>[2x]QEDEDGDYEELVLALRSEEDGLAEAPEHGTTATFHRCAKDPWRLPGTYVVVLKEETHLSQSERTARRLQAQAARRGYLTKILHVFHGLLPGFLVKMSGDLLELALKLPHVDYIEEDSSVFAQSIPWNLERITPPRYRADEYQPPDGGSLVEVYLLDTSIQSDHREIEGRVMVTDFENVPEEDGTRFHRQASKCDSHGTHLAGVVSGRDAGVAKGASMRSLRVLNCQGKGTVSGTLIGLEFIRKSQLVQPVGPLVVLLPLAGGYSRVL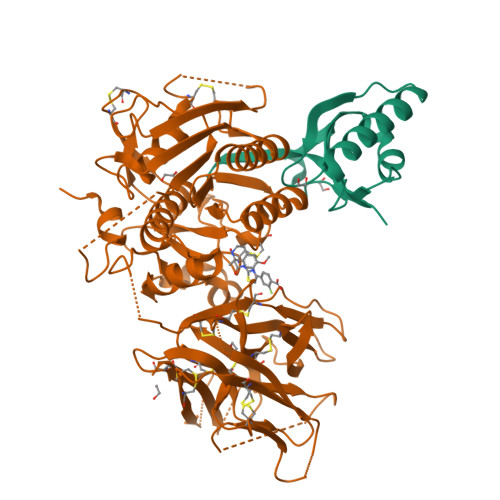NAACQRLARAGVVLVTAAGNFRDDACLYSPASAPEVITVGATNAQDQPVTLGTLGTNFGRCVDLFAPGEDIIGASSDCSTCFVSQSGTSQAAAHVAGIAAMMLSAEPELTLAELRQRLIHFSAKDVINEAWFPEDQRVLTPNLVAALPPSTHGAGWQLFCRTVWSAHSGPTRMATAIARCAPDEELLSCSSFSRSGKRRGERMEAQGGKLVCRAHNAFGGEGVYAIARCCLLPQANCSVHTAPPAEASMGTRVHCHQQGHVLTGCSSHWEVEDLGTHKPPVLRPRGQPNQCVGHREASIHASCCHAPGLECKVKEHGIPAPQEQVTVACEEGWTLTGCSALPGTSHVLGAYAVDNTCVVRSRDVSTTGSTSEEAVTAVAICCRSRHLAQASQELQKGNSADIQHSGGRSSLEGPRFEGKPIPNPLLGLDSTRTGHHHHHH(E)-5-(1-(2-CARBAMIMIDOYLHYDRAZONO)ETHYL)-N-(1H-INDOL-6-YL)-1H-INDOLE-2-CARBOXAMIDE 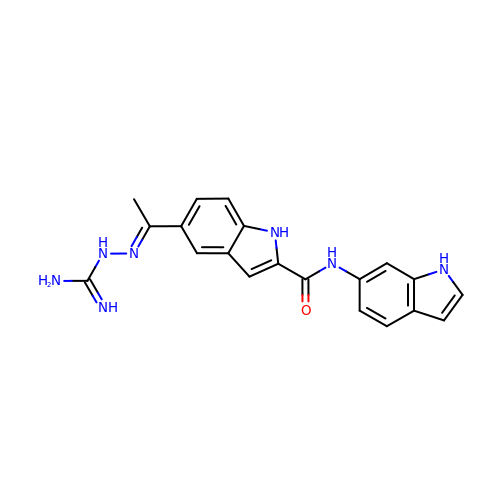| C20 H19 N7 O | STGJVWUQAFPAMH-KBKYJPHKSA-N> GSHMGGELKTVTLSKMKQSLGISISGGIESKVQPMVKIEKIFPGGAAFLSGALQAGFELVAVDGENLEQVTHQRAVDTIRRAYRNKAREPMELVVRVPGPSGSAYGSVKAYTNFDAERDALNIETAIKTKGVDEVTIVNILTNRSNEQRQDIAFAYQRRTKKELASALKSALSGHLETVILGLLKTPAQYDASELKASMKGLGTDEDSLIEIICSRTNQELQEINRVYKEMYKTDLEKDIISDTSGDFRKLMVALAK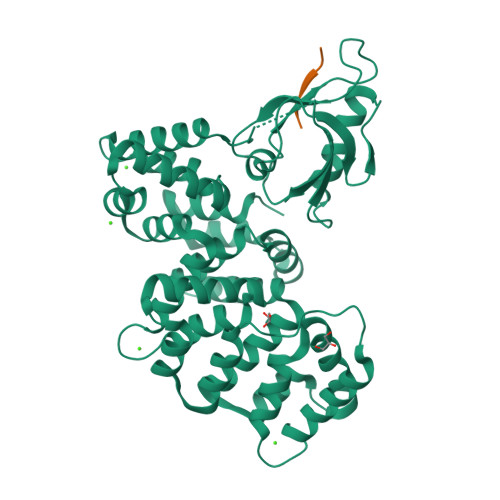GRRAEDGSVIDYELIDQDARDLYDAGVKRKGTDVPKWISIMTERSVPHLQKVFDRYKSYSPYDMLESIRKEVKGDLENAFLNLVQCIQNKPLYFADRLYDSMKGKGTRDKVLIRIMVSRSEVDMLKIRSEFKRKYGKSLYYYIQQDTKGDYQKALLYLCGGDD;> ATKDKKITTV>[3x]MANVDEAILKRVKGWAPYVDAKLGFRNHWYPVMFSKEINEGEPKTLKLLGENLLVNRIDGKLYCLKDRCLHRGVQLSVKVECKTKSTITCWYHAWTYRWEDGVLCDILTNPTSAQIGRQKLKTYPVQEAKGCVFIYLGDGDPPPLARDTPPNFLDDDMEILGKNQIIKSNWRLAVENGFDPSHIYIHKDSILVKDNDLALPLGFAPGGDRKQQTRVVDDDVVGRKGVYDLIGEHGVPVFEGTIGGEVVREGAYGEKIVANDISIWLPGVLKVNPFPNPDMMQFEWYVPIDENTHYYFQTLGKPCANDEERKKYEQEFESKWKPMALEGFNNDDIWAREAMVDFYADDKGWVNEILFESDEAIVAWRKLASEHNQGIQTQAHVSGLEHHHHHH;>MNQIWLKVCAASDMQPGTIRRVNRVGAAPLAVYRVGDQFYATEDTCTHGIASLSEGTLDGDVIECPF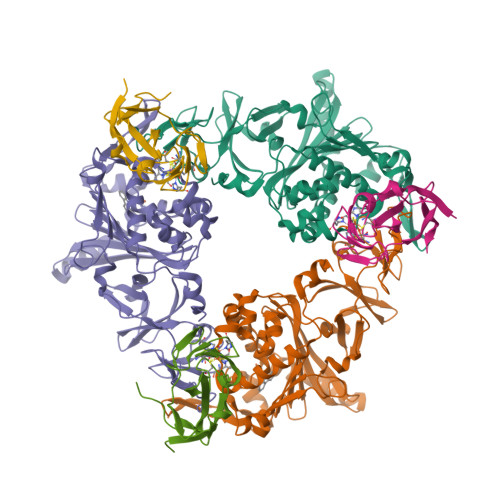HGGAFNVCTGMPASSPCTVPLGVFEVEVKEGEVYVAGEKKLEHHHHHH[3x]> QLICVNENGGCEQYCSDHTGTKRSCRCHEGYSLLADGVSCTP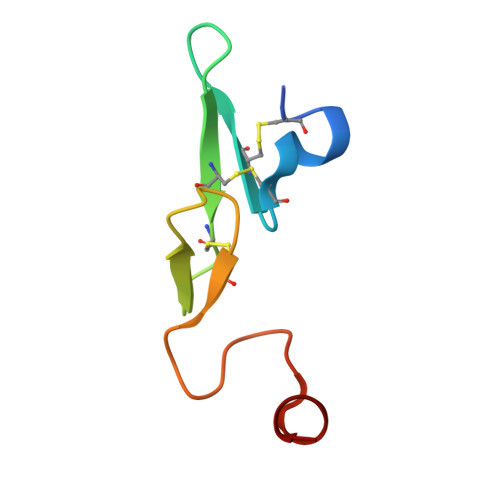TVEYPCGKIPILEKR>[2x]MDNRQFLSLTGVSKVQSFDPKEILLETIQGVLSIKGEKLGIKHLDLKA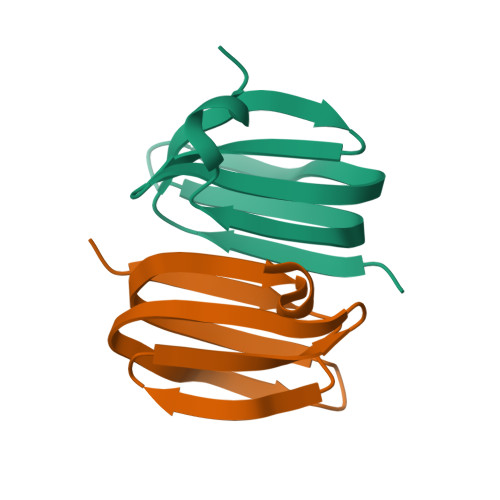GQVEVEGLIDALVYPLEHHHHHH> MLLARMNPQVQPENNGADTGPEQPLRARKTAELLVVKERNGVQCLLAPRDGDAQPRETWGKKIDFLLSVVGFAVDLANVWRFPYLCYKNGGGAFLIPYTLFLIIAGMPLFYMELALGQYNREGAATVWKICPFFKGVGYAVILIALYVGFYYNVIIAWSLYYL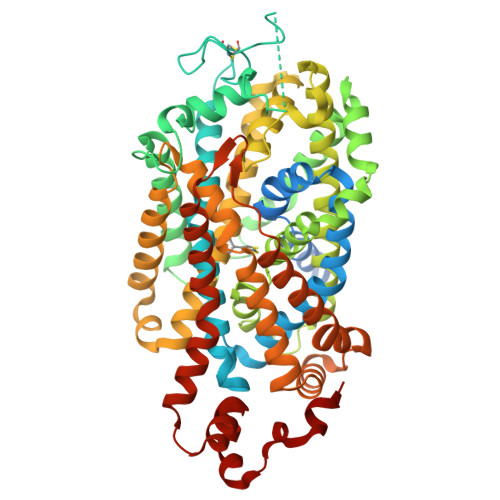FSSFTLNLPWTDCGHTWNSPNCTDPKLLNGSVLGNHTKYSKYKFTPAAEFYERGVLHLHESSGIHDIGLPQWQLLLCLMVVVIVLYFSLWKGVKTSGKVVWITATLPYFVLFVLLVHGVTLPGASNGINAYLHIDFYRLKEATVWIDAATQIFFSLGAGFGVLIAFASYNKFDNNCYRDALLTSSINCITSFVSGFAIFSILGYMAHEHKVNIEDVATEGAGLVFILYPEAISTLSGSTFWAVVFFVMLLALGLDSSMGGMEAVITGLADDFQVLKRHRKLFTFGVTFSTFLLALFCITKGGIYVLTLLDTFAAGTSILFAVLMEAIGVSWFYGVDRFSNDIQQMMGFRPGLYWRLCWKFVSPAFLLFVVVVSIINFKPLTYDDYIFPPWANWVGWGIALSSMVLVPIYVIYKFLSTQGSLWERLAYGITPENEHHLVAQRDIRQFQLQHWLAI>GMDNRELWKVLNVDLEKHDEFLAPVPAVYRELFLNRPNRPRAMAYFDAVVGDIHGIRVHELYNLKQEGKKVFATFCVYVPEEIINATGSACIGLCGGAQYTVPAGETVLPRNLCPLIKSAMGFKIERICPYFQVADYVVGETTCDGKKKAWEILNEYIPVYVMELPQKKEERDRKFWEEEIKDFAQFVEEKTGVKLNAENLRAGIEKINKKRKALKRLSDLRKHNPAPIHGLDVLLINQLAFFDDPERFATKVNELCDELEERVAKGEGVVSKDAPRILITGTPQPIPHWKIHALIEGAGGVVVGEETCIGERYFKDLVEPAADVEGMLKNIAARSLKVNCACFTPNTGRLEDILSMV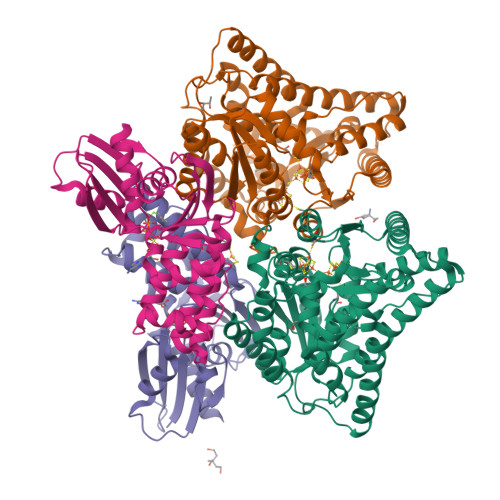QKLQVDGVIHYSLQFCQPYGVESYLVGRELERRNIPFLKLESDFSEEDQGQLKTRIEAFLEMIK[4x];>[4x]MFAGLDLGSTNSKLVIIKEDGSYTFKVVPTRYEPVKAGELLLKNTGEIRNLVVTGYGRVAFNRGKVVTEITCQARGCHELFPEVDYILDLGGQDAKIIKKDGQGRVVNFLMNDKCAAGTGRFLEIILTAIGDDYRDEDLINEENAVPINSMCTVFAESEVISLLARGTSKRAVIAGLFKTTAKRLAKFAESLGKPRKLIFTGGGAKYPALRLFLQKEMGVEVVVPPEPSVTAALGAALIARET The Mex67–Mtr2 complex (NXF1–NXT1 in metazoans and small bristles in Drosophila melanogastor) is the principal mRNA-export factor in Sacccharomyces cerevisiae. Mex67/NXF1 is a modular protein constructed from four domains: an RNA-recognition motif (RRM) domain, a leucine-rich repeat (LRR) domain, a nuclear transport factor 2-like (NTF2L) domain and an ubiquitin-associated (UBA) domain. Mtr2 is a ∼15–20 kDa protein that also has an NTF2-like fold and forms a tight heterodimeric complex with the Mex67 NTF2L domain.

The ctMex67UBA fold was based on three α-helices similar to those seen in H. sapiens and S. cerevisiae and there was a hydrophobic pocket in an equivalent position to where a FG nucleoporin peptide binds in the H. sapiens homologue, indicating that ctMex67UBA probably also interacts with FG nucleoporins in a similar fashion. The ctMex67 UBA domain contained a four-residue C-terminal extension compared with the H. sapiens homologue that formed interactions with the end of α1 in seven copies of the eight in the asymmetric unit and which might contribute to thermostability. The UBA domains and Mtr2/NXT1 showed a high level of structural conservation (Cα r.m.s.d. < 0.8 Å), whereas the NTF2L domain showed the greatest variation (Cα r.m.s.d. = 1.9 Å). The UBA domain showed the greatest conservation (29% sequence identity over 55 residues), whereas the RRM domain had the lowest (15% identity over 73 residues).

>[8x]SNAATKAQLIAEVSRRTGMNVEYSQMCLTGAANWNLELALQSFEQQKANVPPEAFISQPQV Here we report the use of single particle cryo-EM to identify multiple proteins from three enriched heterogeneous fractions prepared from human liver mitochondrial lysate. Using this approach, we were able to simultaneously identify and solve cryo-EM structures of nine different human mitochondrial enzymes: short chain acyl-CoA dehydrogenase (SCAD), medium chain acyl-CoA dehydrogenase (MCAD), isovaleryl-CoA dehydrogenase (IVD), delta (3, 5)-delta dienoyl-CoA isomerase (ECH1), aspartate aminotransferase (GOT2), glutamate dehydrogenase (GLUD1), mitochondrial superoxide dismutase 2 (SOD2), catalase (CAT), and mitochondrial aldehyde dehydrogenase (ALDH2). Functionally, the three acyl-CoA dehydrogenases—SCAD, MCAD and IVD—are involved in beta oxidation and amino acid catabolism. Finally, SOD2, CAT, and ALDH2 are all involved in clearing toxic byproducts of oxidative respiration.

MCAD has a relatively broad substrate specificity but has highest activity with octanoyl-CoA. An FAD cofactor-bound MCAD structure was resolved at 2.69 Å using 18,616 single particle cryo-EM projections. Consistent with previous crystal structures of human and pig MCAD, our structure is a tetramer consisting of a dimer of dimers. The overall fold is similar to that of SCAD. Each monomer is made up of three domains; an N-terminal α-helical bundle, a β-sheet core, and a C-terminal α-helical domain. Residues T121, T124, A125, L128, F277, T280, R281, V284, Y398, Y400, and the catalytic residue E401 form the binding cavity. The substrate accommodation in the binding cavity is determined by a network of hydrogen bonds among residues Q120, T121, Q242, Y398, and Y400. In the MCAD structure, helix 4 and helix 6 are shifted relative to the corresponding SCAD structure. These two helices form the edge of the substrate cavity, resulting in a deeper substrate-binding pocket in the MCAD structure. Several of the mutations identified in newborn screening of MCAD deficiency, including the most common K329E mutation, are not within the active site but instead appear to be involved in the dimer–dimer interface, which would disrupt assembly and limit activity.

>[4x]MAAGFGRCCRVLRSISRFHWRSQHTKANRQREPGLGFSFEFTEQQKEFQATARKFAREEIIPVAAEYDKTGEYPVPLIRRAWELGLMNTHIPENCGGLGLGTFDACLISEELAYGCTGVQTAIEGNSLGQMPIIIAGNDQQKKKYLGRMTEEPLMCAYCVTEPGAGSDVAGIKTKAEKKGDEYIINGQKMWITNGGKANWYFLLARSDPDPKAPANKAFTGFIVEADTPGIQIGRKELNMGQRCSDTRGIVFEDVKVPKENVLIGDGAGFKVAMGAFDKTRPVVAAGAVGLAQRALDEATKYALERKTFGKLLVEHQAISFMLAEMAMKVELARMSYQRAAWEVDSGRRNTYYASIAKAFAGDIANQLATDAVQILGGNGFNTEYPVEKLMRDAKIYQIYEGTSQIQRLIVAREHIDKYKN> MVGLTTLFWLGAIGMLVGTLAFAWAGRDAGSGERRYYVTLVGISGIA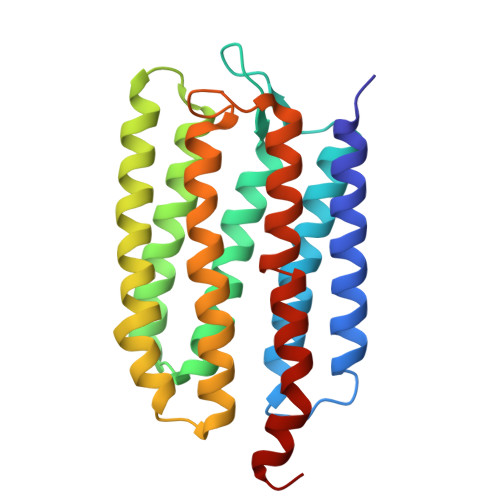AVAYVVMALGVGWVPVAERTVFAPRYIDWILTTPLIVYFLGLLAGLDSREFGIVITLNTVVMLAGFAGAMVPGIERYALFGMGAVAFLGLVYYLVGPMTESASQRSSGIKSLYVRLRNLTVILWAIYPFIWLLGPPGVALLTPTVDVALIVYLDLVTKVGFGFIALDAAATLRAEHGE Deoxyribonucleotides, the building blocks for DNA biosynthesis, are produced in the cell from ribonucleotide precursors by ribonucleotide reductase (RNR). The best characterized of all RNRs is the class Ia enzyme from Escherichia coli that employs a di-iron-tyrosyl-radical cofactor to initiate chemistry and requires two dimeric protein subunits for enzymatic activity. As a central controller of nucleotide metabolism, RNR uses multiple allosteric mechanisms to maintain the balanced deoxyribonucleoside triphosphate (dNTP) pools that are required for accurate DNA replication. Briefly, the binding of (d)NTP effectors to an allosteric specificity site in α2 influences the preference of RNR for its four nucleoside diphosphate (NDP) substrates.

We have utilized an α4β4 crystal form of the E. coli class Ia RNR (right) to obtain structures of all four substrate/specificity effector pairs (CDP/dATP, UDP/dATP, ADP/dGTP or GDP/TTP) bound to the α2 subunit. Each model consists of two α2 dimers, two β2 dimers, and activity effector dATP in all four allosteric activity sites. Although the α4β4 form of the enzyme cannot turn over substrates due to abrogation of the radical transfer pathway, the substrate and effector binding sites are not affected. Whereas high levels of dATP inhibit class Ia RNR, at lower levels, dATP promotes CDP or UDP reduction. The remaining interactions with loop 2 are distinct for each substrate/effector pair. dATP, which preferentially increases RNR activity for CDP and UDP substrates, makes two hydrogen bonds with loop 2. The backbone amide and carbonyl of Ser293 are in position to hydrogen bond to N1 and N6, respectively, of the adenine base of dATP. These hydrogen bonds hold Ser293 in place and position the adjacent Gln294 in to a conformation that points into the substrate-binding site. In this conformation, Gln294 can form a hydrogen bond with O2 of CDP or UDP. There is no difference in substrate positioning between CDP and UDP, as the unique positions of the pyrimidine ring (N2 and N4/O4) are not involved in any contacts with the protein. Each substrate/effector bound α4β4 structure reveals a closing of the (β/α)10 barrel around the bound substrate that is not observed in the absence of substrate.

>[4x]MNQNLLVTKRDGSTERINLDKIHRVLDWAAEGLHNVSISQVELRSHIQFYDGIKTSDIHETIIKAAADLISRDAPDYQYLAARLAIFHLRKKAYGQFEPPALYDHVVKMVEMGKYDNHLLEDYTEEEFKQMDTFIDHDRDMTFSYAAVKQLEGKYLVQNRVTGEIYESAQFLYILVAACLFSNYPRETRLQYVKRFYDAVSTFKISLPTPIMSGVRTPTRQFSSCVLIECGDSLDSINATSSAIVKYVSQRAGIGINAGRIRALGSPIRGGEAFHTGCIPFYKHFQTAVKSCSQGGVRGGAATLFYPMWHLEVESLLVLKNNRGVEGNRVRHMDYGVQINKLMYTRLLKGEDITLFSPSDVPGLYDAFFADQEEFERLYTKYEKDDSIRKQRVKAVELFSLMMQERASTGRIYIQNVDHCNTHSPFDPAIAPVRQSNLCLEIALPTKPLNDVNDENGEIALCTLSAFNLGAINNLDELEELAILAVRALDALLDYQDYPIPAAKRGAMGRRTLGIGVINFAYYLAKHGKRYSDGSANNLTHKTFEAIQYYLLKASNELAKEQGACPWFNETTYAKGILPIDTYKKDLDTIANEPLHYDWEALRESIKTHGLRNSTLSALMPSETSSQISNATNGIEPPRGYVSIKASKDGILRQVVPDYEHLHDAYELLWEMPGNDGYLQLVGIMQKFIDQSISANTNYDPSRFPSGKVPMQQLLKDLLTAYKFGVKTLYYQNTRDGAEDAQDDLVPSIQDDGCESGACKI;>AYTTFSQTKNDQLKEPMFFGQPVNVARYDQQKYDIFEKLIEKQLSFFWRPEEVDVSRDRIDYQALPEHEKHIFISNLKYQTLLDSIQGRSPNVALLPLISIPELETWVETWAFSETIHSRSYTHIIRNIVNDPSVVFDDIVTNEQIQKRAEGISSYYDELIEMTSYWHLLGEGTHTVNGKTVTVSLRELKKKLYLCLMSVNALEAIRFYVSFACSFAFAERELMEGNAKIIRLIARDEALHLTGTQHMLNLLRSGADDPEMAEIAEECKQECYDLFVQAAQQEKDWADYLFRDGSMIGLNKDILCQYVEYITNIRMQAVGLDLPFQTRSNPIPWINTWLVSDNVQVAPQEVEVSSYLVGQIDSEVDTDDLSNFQL[4x]> GLVPRGSHMSGAT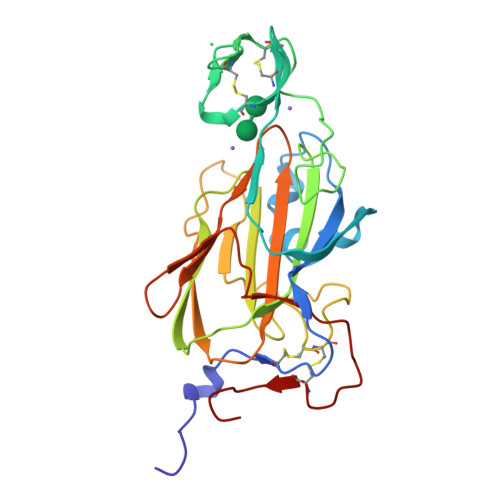EACLPAGQRKSGMNINFYQYSLKDSSTYSNAAYMAYGYASKTKLGSVGGQTDISIDYNIPCVSSSGTFPCPQEDSYGNWGCKGMGACSNSQGIAYWSTDLFGFYTTPTNVTLEMTGYFLPPQTGSYTFSFATVDDSAILSVGGSIAFECCAQEQPPITSTNFTINGIKPWDGSLPDNITGTVYMYAGYYYPLKVVYSNAVAWGTLPISVELPDGTTVSDNFEGYVYSFDDDLSQSNCTIPDPSIH>LTAKHRPSVVWLHNAECVGCTEAAIRTIKPYIDALILDTISLDYQETIMAAAGEAAEAALHQALEGKDGYYLVVEGGLPTIDGGQWGMVAGHPMIETTKKAAAKAKGIICIGTCSAYGGVQKAKPNPSQAKGVSEALGVKTINIPGCPPNPINFVGAVVHVLTKGIPDLDENGRPKLFYGELVHDNCPRLPHFEASEFAPSFDSEEAKKGFCLYELGCKGPVTYNNCPKVLFNQVNWPVQAGHPCLGCSEPDFWDTMTPFYEQG[3x];>[3x]ASWSHPQFEKGASGAAESKPTPQSTFTGPIVVDPITRIEGHLRIMVEVENGKVKDAWSSSQLFRGLEIILKGRDPRDAQHFTQRACGVCTYVHALASSRCVDDAVKVSIPANARMMRNLVMASQYLHDHLVHFYHLHALDWVDVTAALKADPNKAAKLAASIAPARPGNSAKALKAVQDKLKAFVESGQLGIFTNAYFLGGHKAYYLPPEVDLIATAHYLEALHMQVKAASAMAILGGKNPHTQFTVVGGCSNYQGLTKDPLANYLALSKEVCQFVNECYIPDLLAVAGFYKDWGGIGGTSNYLAFGEFATDDSSPEKHLATSQFPSGVITGRDLGKVDNVDLGAIYEDVKYSWYAPGGDGKHPYDGVTDPKYTKLDDKDHYSWMKAPRYKGKAMEVGPLARTFIAYAKGQ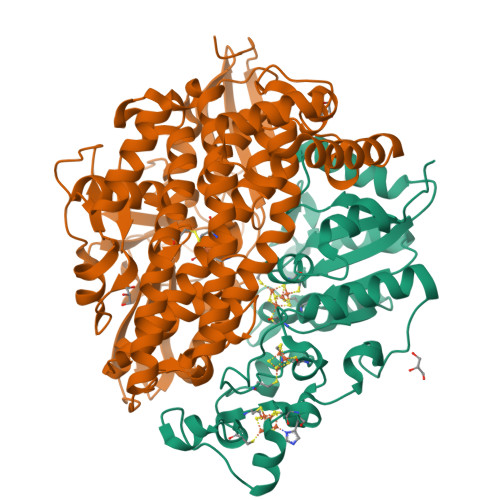PDFKKVVDMVLGKLSVPATALHSTLGRTAARGIETAIVCANMEKWIKEMADSGAKDNTLCAKWEMPEESKGVGLADAPRGALSHWIRIKGKKIDNFQLVVPSTWNLGPRGAQGDKSPVEEALIGTPIADPKRPVEILRTVHAFDPCIACGVH> NKTLAAMKNFAEQYAKRTDTYFCSDLSVTAVVIEGLARHKEELGSPLCPCRHYEDKEAEVKNTFWNCPCVPMRERKECHCMLFLTPDNDFAGDAQDIPMETLEEVKASMA;> MNVGDRVRVTSSVVVYHHPEHKKTAFDLQGMEGEVAAVLTEWQGRPISANLPVLVKFEQRFKAHFRPDEVTLIE;> EAIVGKVTEVNKDTFWPIVKAAGDKPVVLDMFTQWCGPSKAMAPKYEKLAEEYLDVIFLKL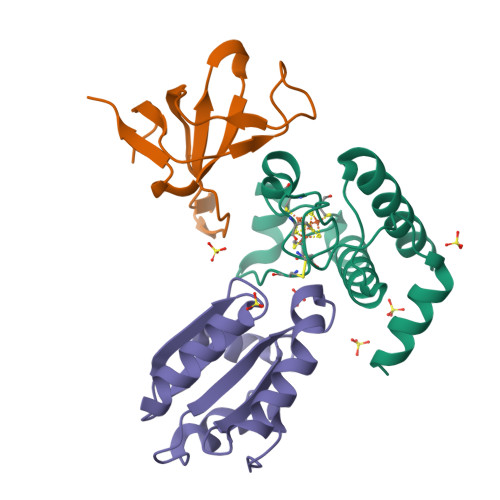DCNQENKTLAKELGIRVVPTFKILKENSVVGEVTGAKYDKLLEAIQAARS> GMIDFTKSKQYTLSIRLSTDGFSFSIYNPINDNSQSLFEKEVDTSLSLTANLKNVFHESDFLSYSYKRVNIMIASKRFTMIPLELFEEEQAELLFYHNHQKRENEIVMYNILKKNNVVIIFGIDKSTYTFLNEQYPEARFYSQSTPLIEYFSIKSRLGNSK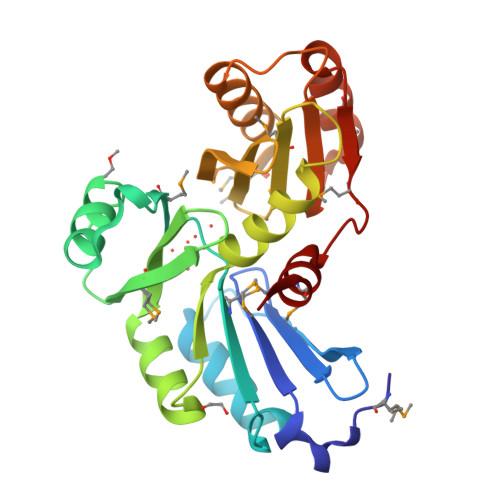KMYASVRKDAIDIYCFERGQLLLANSFECMQTEDRIYYLLYVWKQLEFNQERDELHLTGTLSDKETLMNELKKFILQVFIMNPANNIDMQALLTCE> MELLGEYVGQEGKPQKLRVSCEAPGDGDPFQGLLSGVAQM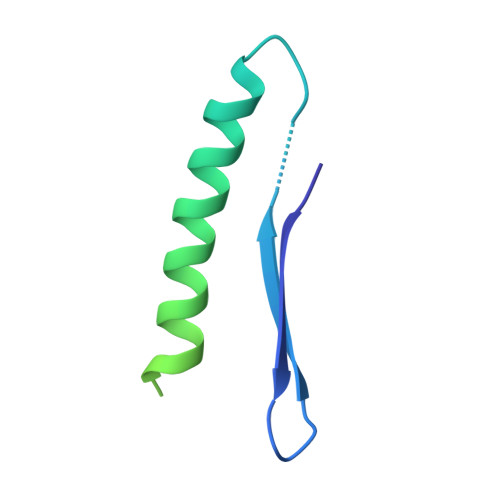KDMVTELFDPLVQGEVQHRVAAAPDEDLDGDDEDDAEDENNIDNRTNFDGPSAKRPKTPSHHHHHH>FLGALFRALSRLL[102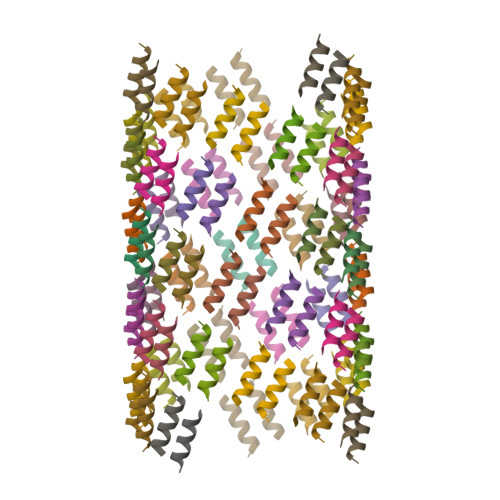x]> GIEDLITEVAQGALTLSLPKQQDSLPDTKASGPAHSKEVPALTAVETGATNPLVPSDTVQTRHVIQRRSRSESTIESFFARGACVAIIEVDNEEPTTRAQKLFAMWRITYKDTVQLRRKLEFFTYS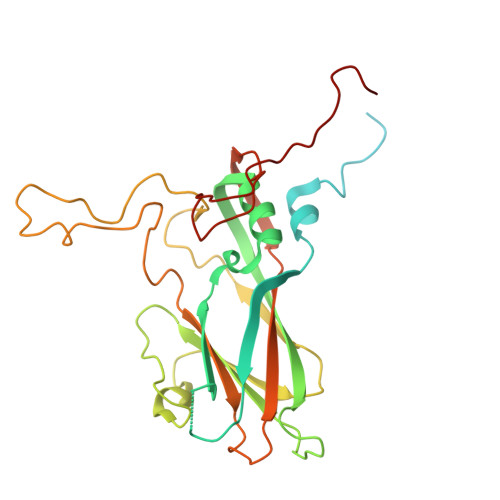RFDMELTFVVTANFTNTNNGHALNQVYQIMYIPPGAPTPKSWDDYTWQTSSNPSIFYTYGAAPARISVPYVGLANAYSHFYDGFAKVPLKTDANDQIGDSLYSAMTVDDFGVLAIRVVNDHNPTKVTSKVRIYMKPKHVRVWCPRPPRAVPYYGPGVDYKDNLNPLSEKGLTTY>MAKLETVTLGNIGKDGKQTLVLNPRGVNPTNGVASLSQAGAVPALEKRVTVSVSQPSRNRKNYKVQVKIQNPTACTANGSCDPSVTRQAYADVTFSFTQYSTDEERAFVRTELAALLASPLLIDAIDQLNPAY[180x];> MPKLPRGLRFGADNEILN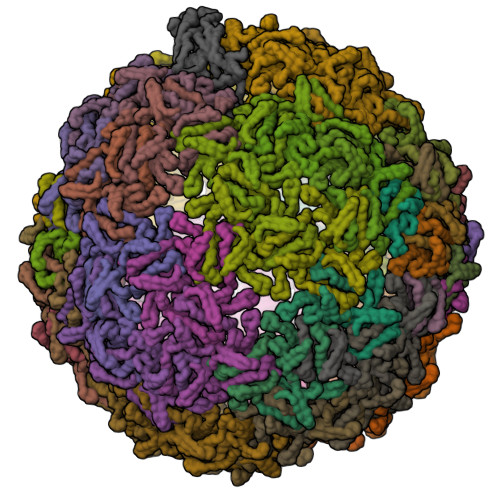DFQELWFPDLFIESSDTHPWYTLKGRVLNAHLDDRLPNVGGRQVRRTPHRVTVPIASSGLRPVTTVQYDPAALSFLLNARVDWDFGNGDSANLVINDFLFRTFAPKEFDFSNSLVPRYTQAFSAFNAKYGTMIGEGLETIKYLGLLLRRLREGYRAVKRGDLRALRRVIQSYHNGKWKPATAGNLWLEFRYGLMPLFYDIRDVMLDWQNRHDKIQRLLRFSVGHGEDYVVEFDNLYPAVAYFKLKGEITLERRHRHGISYANREGYAVFDNGSLRPVSDWKELATAFINPHEVAWELTPYSFVVDWFLNVGDILAQQGQLYHNIDIVDGFDRRDIRLKSFTIKGERNGRPVNVSASLSAVDLFYSRLHTSNLPFATLDLDTTFSSFKHVLDSIFLLTQRVKR>[4x]MHHHHHHLKNGMRPIHPGEILREEFQKEMGFSAAALARALGVATPTVNNILRERGGVSADMALRLSICLDTTPEFWLNLQTAFDLRTAEQQHGDEIIGSVQRLVA

GraTA (Growth rate affecting Toxin–Antitoxin) is a type II TA module recently discovered in Pseudomonas putida. By sequence similarity, GraTA is most closely related to the higBA TA family. Here we show that GraA does not contain unstructured regions and forms a globular dimer while the toxin GraT contains an N-terminal intrinsically disordered region that is key for transcriptional regulation of the graTA operon as well as for the RNase activity of GraT. GraA binds tightly to the graTA operator and GraT prevents this interaction through steric interference from its N-terminal disordered region.

The crystal structure of GraA was determined at 1.96 Å. The protein was completely traced and, in contrast to other antitoxins, does not contain an intrinsically unfolded domain. GraA forms a homo-dimer (from now on referred to as GraA2). The GraA monomer consists of one long and four short (2–3 turns) α-helices, of which helices α2 and α3 form a helix-turn-helix (HTH) motif. Helix α5 extends over seven turns to form a dimerization unit and its C-terminus (after a kink) also caps over the globular domain of the other monomer. The dimerization interface of GraA2 is mainly stabilized by hydrophobic interactions. The helix-turn-helix DNA binding motif, comprising residues from 25 to 45, presents a positively charged surface. The separation between the two HTH motifs in the dimer, measured as the distance between the centers of mass of both α3 helices, is 33.8 Å. The closest homolog with known structure for GraA is C. burnetti HigA (backbone root-mean-square deviation (RMSD) of 2.6 Å for residues 4–99 when superimposing monomers). In contrast with most antitoxins, GraA is a fully ordered protein and, in accordance with that, is also uncommonly stable and not degraded by Lon or Clp20.> MSFEGKIALVTGASRGIGRAIAELLVERGACVIGTATSEKGAEAISAYLGENGKGLMLNVVDPTSIDTVLATIR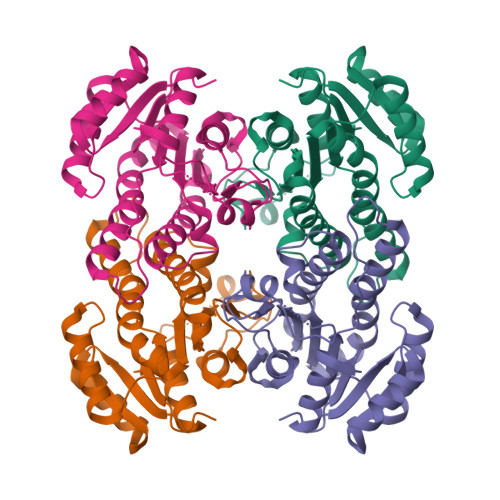AEFGEVDILVNNAGITRDNLLMRMKDDEWQDIIDTNLTSVFRLSKAVMRAMMKKRFGRIITIGSVVGTMGNAGQVNYAAAKAGVIGFSKSLAREVASRGITVNVVAPGFIETDMTRTLTDDQRAGILAQVPANRLGDAKEIASAVAFLASDEASYISGETLHVNGGMYMI>AEETSFVFSKFKPLEPNLILQGDALVTVAGVLQLTNVDKNGVPEPSSLGRATYSAPINIWDSATGLVASFATSFRFTIYAPNIATIADGLAFFLAPVASAPDSGGGFLGLFDSAVSGSTYQTVAVEFDTYENTVFTDPPYTHIGFDVNSISSIKTVKWSLANGEAAKVLITYNSAVKLLVASLVYPSSKTSFILADIVDLSSVLPEWVRVGFSAATGASGGKIETHDVFSWSFASKLAGXXTKDSSFLDGG[2x];>AEETSFVFSKFKPLEPNLILQGDALV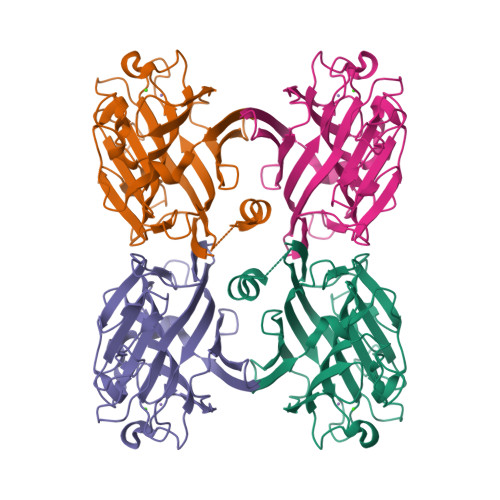TVAGVLQLTNVDSNGVPEPSSLGRATYSAPINIWDSATGLVASFATSFRFTIYAPNIATIADGLAFFLAPVASAPDSGGGFLGLFDSAVGDTTYQTVAVEFDTYENTVFTDPPYTHIGFDVNSISSIKTVKWSLANGEAAKVLITYNSAVKLLVASLVYPSSKTSFILADIVDLSSVLPEWVRVGFSAATGASKGYIETHDVFSWSFASKLAG[2x]> MPISPIETVPVKLKPGMDGPKVKQWPLTEEKIKALVEICTEMEKEGKISKIGPENPYNTPVFAIKKKDSTKWRKLVDFRELNKRTQDFWEVQLGIPHPAGLKQKKSVTVLDVGDAYFSVPLDKDFRKYTAFTIPSINNETPGIRYQYNVLPQGWKGSPAIFQCSMTKILEPFRKQNPDIVIYQYMDDLYVGSDLEIGQHRTKIEELRQHLLRWGFTTPDKKHQKEPPFLWMGYELHPDKWTVQPIVLPEKDSWTVNDIQKLVGKLNWASQIYAGIKVRQLCKLLRGTKALTEVVPLTEEAELELAENREILKEPVHGVYYDPSKDLIAEIQKQGQGQWTYQIYQEPFKNLKTGKYARMKGAHTNDVKQLTEAVQKIATESIVIWGKTPKFKLPIQK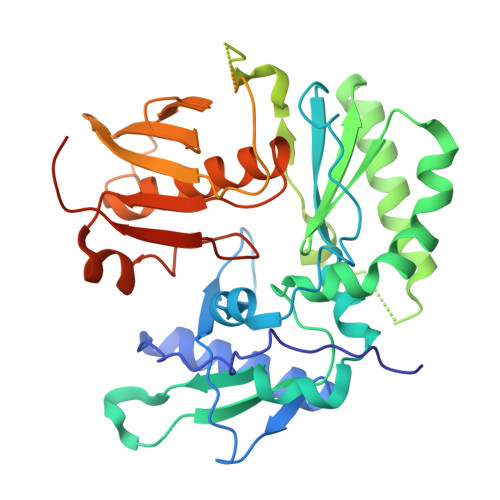ETWEAWWTEYWQATWIPEWEFVNTPPLVKLWYQLEKEPIIGAETF>[2x]MLKKNETFYTYCSYKKEDGYVRRGLIVLPTLHIAMFAPFLLALLVPFFYKCIRSLHVGWFVFPLPIALFVYFLSYIDDVRNDEVIRATMPWIPSLRISFDAYVDGLSLLFALLITGIGSLVVLYSIYYLQKGKEPLGNFYVYLLLFMGAMLGVVLSDHLIALYMFWELTSISSFLLIAYWFKRDRSRYGAQKSMLITMFGGLLMLGGFVALAIAGGTY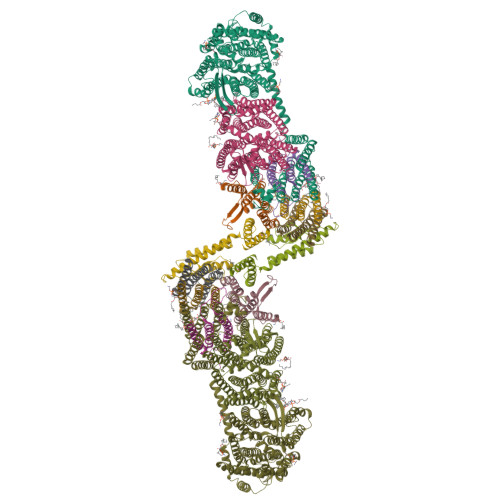NIRELVHTPLTEHPLFIPALVLILFGAFTKSAQFPFYIWLPDAMEAPTPVSAYLHSATMVKAGIYVIARLTPIFAVSSVWVWTVALVGLVTLCWASFLASKQTDLKAILAYSTVSQLGLITSLLGIGGLSFHYDGMGENVFMVAVLAAIFHLFNHATFKGSLFMVVGIVDHETGTRDIRRLGGLMTIMPITFTIALIGSLSMAGLPPFNGFLSKEMFFTAMLRAKDVAGWAVILPVVAWVASIFTFLYSALLVSRTFFGTYKPHVLKKEAHEAPFGMLIAPIVLASLVVFIGFVPNVLSDSVLAPAVYAVLYGLFAPNEALDVHISHWHGFTPELFMTIGVLLFGLVLYRTFPKWKKIYYRLSERMSLNFFYDQSFVWMERGARSFISRVMNGSMRTYLMYIFTSLVALLLFTIGWHEQWHIDLSRLAHVRVYEVVLAIGILAATVTTVIAKSRLTAIVSLGAVGYAVALFFVLFRAPDLALTQLVIETISVALFLLCFYHLPKFTQKQESVRFHLGNALVSLAVGMTMSIIAFLAYAGKHFDSISQYYVDNTYEKAAGKNMVNVILVDFRGFDTLFEICVLAIAALGIYAMVKLRLAKEEER;>MKRNDVILRTTTAVVTPIIVLFSVQLFFAGHYYPGGGFIGGLMTAGAIVLLLLAFDIETVRKMVPINYKWLVAIGLLFAVGTGMSSMFLDRPFLTHAYKYVHLPLLDHTSLHTAVLFDLGVYFVVVGVTMIIIETIGESD[2x];>[2x]MELLMIVVIGCLFAAATYLLLSKSLLRIIIGTGLLSHGAHLLLLTMGGLKAGAPPLLGEKASRYVDPLPQALILTAIVISFGVTAFFLVLAYRSYQEIGTDHMEGMKGD;>[2x]MSNLLLLPIVIPLVTAIVLIFFPKHVFWQRVVSLAATVGLVVASGALLHRVHTDGIQTLNVGNWPAPFGITLVSDSLSALLVLTTSIIALACLVYSFYAIGHKRETFYYYSFFQFLIVGVNGAFTTGDLFNLFVFFEVMLMSSYVLLVLGGTKIQLRETIKYTLVNVISSALFVVAVAYLYAVTGTLNMAHLADRINALGSSPILTVIAVLFIIVFGLKGAIFPLYFWLPGAYYAPPTPVLALFGGLLTKVGVYSILRTFTLLFTHDAAYTHTLLAWLALGTIIIGVIGAVAYNDMRYIVIYNIIAAVGVMIFGISIMTPESVEGTIFYLLQDMVMKAMLFLFVGIIFSITRSNDIRSFSGLITSYPLLGWAFFIAALSLAGIPPLSGFIGKLLIVKASFDAQLIFEAIVILLSSLLVLYSVMKIFMNGFWGEKKGFEQKQVDGRLFPVLFLLVLSVAYGIGIEFVRPFVLDAVNVLVDPSMYIEAVLKE;>MAFQILLNVILAFVWMFLTVSFDGASFLVGYMIGLFILFILRRFFHSRFYLVPVFVIIKLLFIFFKELILSNIAVAKVVMQRSLTIQPAIFALPTELKKEWEITVLAMLITLTPGTLVLDVSDDGSTLYIHALNSPDVHEAIESIKQSFEKTIMEVSK[2x];>[2x]MMLNIALVILSLAMVGFLYRVVKGPSTADRIIALDAMGITLAGIVAIVSMLLNTSAFLDVILLIGILAFVGTVAFAKFLEKGVVIERGNDR;>MSSNVGTIANALVVVLILLGAVLTLLSAVGAIRLPDVYTRSHAISKSTTLGIMCILLGAFLHFFIENNHFNSRLLLGIVFIFMTSPVAAHLISRAAYYANVERWEGTVRDDLKQKAGGK[2x]>[2x]MGTKIIGTGVYLPKNVLTNFDLEKIVDTSDEWITTRTGIKER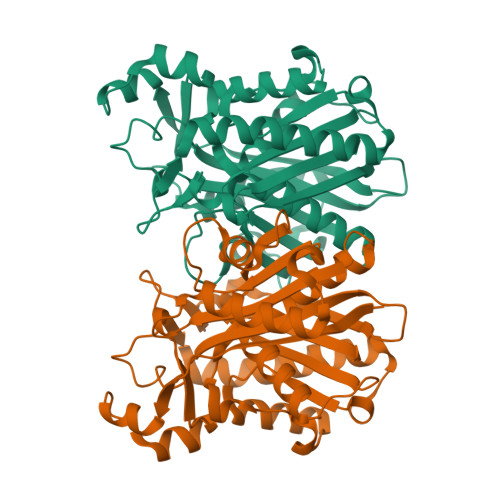RIAKEETITYMATQAAKEALREANLSPEELDLIILATLTPQKRFPSTACLVQAQLKAKGVYAFDISAACSGFIYALDIADSFIKSGKAKNVLVIGAEKLSEAVDWEDRSTCVLFGDGAGAVVVTRSEDKSDILATRMYAEGSLEELLHADNCGYIRMKGRELFKVAVRSMEEVCREVLEKAGVKPEEVSLVIPHQANVRIINALAEKLNIPKEKVFVNIQKYGNTSAASIPIALHEAIKEGKVKRGDLILMTAMGGGLTWGAVLLRY>GMCQ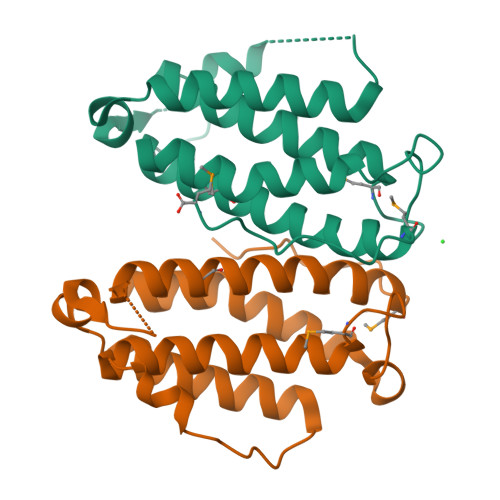SNQIVSHFLSHRNVTNELAEKISKDHYSYKPAETSMSAEELVKHILTSFHLFANVIKEGNASPFQNKQEETETDLNVLAKTYTEKTVAILEQLTEEQLDREIDLTSAFGRKVTGRALLQLAMEHEIHHKGNLFVYVREMGHTELPFYQQRM[2x]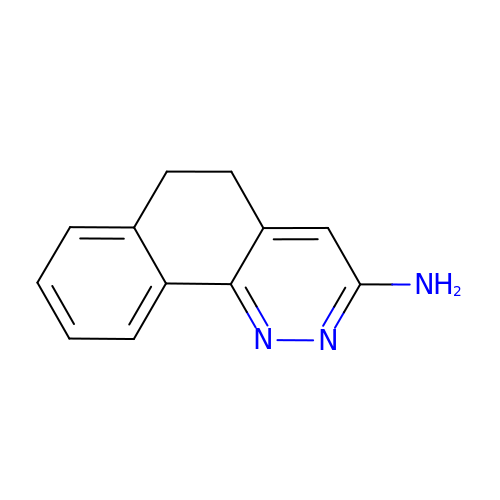5,6-Dihydro-benzo[H]cinnolin-3-ylamine | C12 H11 N3 | QKVREUJWFZJEJK-UHFFFAOYSA-N>MGQQHLLRFALPAGKKLWPNDLREALAKHDLPPLFFSRDPQTGHAITRAMRNEKRVRGYIEQHGHEPPPPTEEQRANPLAIPGIRIVGSSTWVGILATGERYKPLLEAATLPAIQIVTQRCGRGVGVELEQHTLSIKGLDDPKRYFVRNLVMKRGLTKTAENTTQVASRILSALERQAVAYSLDLPPTAQVDIHVESVVRPRGMRLVTSTGATEQFVGLADVEFYACLDL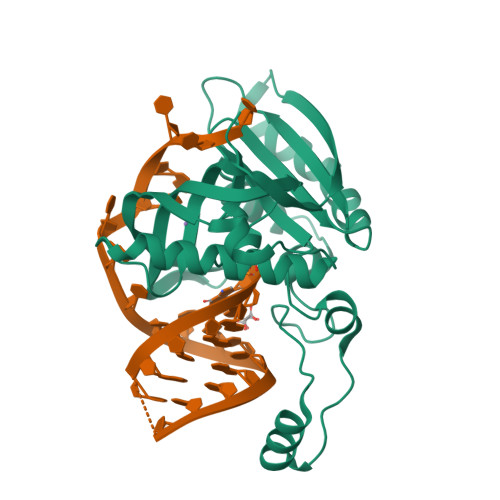KGYWFAGNLTSRGYGRIIADHPAMSTGRYAHHHHHH[2x]>GPLGSMSPPPAESHIILLIQQGSDPKTRIWSDHCSLRSAIEYIVGVYQTNQAVSEKESIDVSRFFNFFDEIYDCVPLVYDRHFRAYIPHEKQWLLHHAQEYLTAARQIP[3x]

Members of the ERH protein family are small proteins found in metazoan, invertebrates as well as plants. Closely related proteins, sharing around 30% sequence identity with human ERH, are also present in Schizosaccharomyces such as S. pombe and in few other fungi. Erh1 cooperates with Mmi1 to target meiosis-specific transcripts for degradation by the nuclear exosome. Erh1 not only suppresses the meiotic program in vegetative cells but also stimulates meiosis progression.

Larger crystals could be obtained by increasing the drop volume, varying the ammonium sulfate concentration and the buffer. From one of these crystals, we could collect a dataset of better quality (see Table 1 for dataset statistics) from which we could determine Erh1 structure by molecular replacement using the structure of human ERH as initial model and refine it to 1.95 Å resolution. Erh1 monomer folds as an α-β protein composed of a four stranded anti-parallel β-sheet and three α helices packed onto the same face of the β-sheet. This fold is similar to that of metazoan ERH (rmsd values of 1.1–1.9 Å over 80 Cα atoms). Three copies (protomers A, B and C) of Erh1 protein are present in the asymmetric unit. Protomers A and B are virtually identical (rmsd values of 0.27 Å over 84 Cα atoms) while protomer C slightly differs as illustrated by its higher rmsd value when compared to the two other chains (1.3–1.4 Å over 84 Cα atoms). The largest differences between protomer C and the two other Erh1 molecules present in the asymmetric unit occur at helix α2 (2.5 Å translation along the helix longitudinal axis), at the hinge between helix α2 and the N-terminal extremity of strand β3, and to a lesser extent on helix α3 (1.3 Å translation). Among the three copies present in the asymmetric unit, protomers B and C associate to form a tight homodimer with a butterfly-like shape while the protomer A forms a similar homodimer with a symmetry-related molecule (rmsd of 1.1 Å over 160 Cα atoms). In the homodimer, the Erh1 β-sheet face from each monomer, which is not packed against α helices, interacts to form a β-barrel. Each monomer engages an area of 850 Å2 mostly formed by hydrophobic residues, which are strongly or strictly conserved within Erh1/ERH orthologues from fungi, plants, insects, worm and animals.(4S,7R)-4-(3-ethoxy-4-hydroxy-5-nitrophenyl)-7-(4-fluorophenyl)-4,6,7,8-tetrahydroquinoline-2,5(1H,3H)-dione 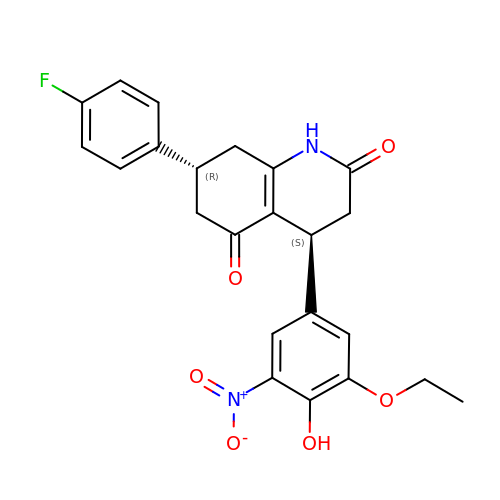| C23 H21 F N2 O6 | ZIQMAORRANWURA-CJNGLKHVSA-N>[2x]SETRLSLEDLFRKDFVLHDPEARWINDTDVVYKSENGHVIKLNIETNATTLLLENTTFVTFKASRHSVSPDLKYVLLAYDVKQIFHYSYTASYVIYNIHTREVWELNPPEVEDSVLQYAAWGVQGQQLIYIFENNIYYQPDIKSSSLRLTSSGKEEIIFNGIADWLYEEELLHSHIAHWWSPDGERLAFLMINDSLVPTMVIPRFTGALYPKGKQYPYPKAGQMNPTIKLYVVNLYGPTHTLELMPPDSFKSREYYITMVKWVSNTKTVVRWLNRAQNISILTVCETTTGACSKKYEMTSDTWLSQQNEEPVFSRDGSKFFMTVPVKQGGRGEFHHIAMFLIQSKSEQITVRHLTSGNWEVIKILAYDETTQKIYFLSTESSPRGRQLYSASTEGLLNRQCISCNFMKEQCTYFDASFSPMNQHFLLFCEGPRVPVVSLHSTDNPAKYFILESNSMLKEAILKKKIGKPEIKILHIDDYELPLQLSLPKDFMDRNQYALLLIMDEEPGGQLVTDKFHIDWDSVLIDMDNVIVARFDGRGSGFQGLKILQEIHRRLGSVEVKDQITAVKFLLKLPYIDSKRLSIFGKGYGGYIASMILKSDEKLFKCGSVVAPITDLKLYASAFSERYLGMPSKEESTYQAASVLHNVHGLKEENILIIHGTADTKVHFQHSAELIKHLIKAGVNYTMQVYPDEGHNVSEKSKYHLYSTILKFFSDCLKE

In this paper, we present the crystal structure of human DPP10, a naturally inactive member of the prolyl oligopeptidase family that belongs to the S9B serine protease subfamily. DPP6 and DPP10 are homologous glycosylated, single-pass type II transmembrane proteins that lack the crucial serine residue of the catalytic triad; instead, DPP6 contains an aspartic acid (Asp712) and DPP10 a glycine (Gly651). The Ca2+ binding proteins (KChIPS) and the dipeptidylpeptidase-like proteins (DPPLs) DPP6 (also known as DPPX) and DPP10 (also known as DPPY) associate with the α-subunits of the Kv4 subfamily to form a ternary complex of approximately 750 kDa containing 12 protein molecules (4 copies of each protein per channel). DPP10 and DPP6 both accelerate the activation and inactivation of Kv4.3 channel gating but with distinct biophysical properties.

The extracellular domain (residues 58–796) was expressed as a secreted protein from insect cells, purified and crystallized in space group P212121 with two molecules in the asymmetric unit. The overall structure of DPP10 is very similar to those of DPP6 and DPP4, with Cα-root-mean-square-deviations (r.m.s.d.) of 1.1 Å (for 646 superimposed atoms) and 1.5 Å (for 578 atoms), respectively. Each subunit consists of two domains: an open (no “Velcro” architecture present) β-propeller (residues 82–517, shown in yellow in Fig. 1) consisting of eight blades each built up by four antiparallel β-strands and a classical α/β-hydrolase fold (residues 517–679 and 707–796; shown in red). Additionally, a small-extended arm formed by three helices is inserted between two β-strands of the hydrolase domain (residues 679–707; shown in blue). In our structure, all these asparagine residues with the exception of Asn-90 were found to be glycosylated and well-defined electron densities were observed for the first sugar residues. Similarly to DPP6, DPP10 has three disulfide bonds in the β-propeller (Cys349-Cys356, Cys465-Cys468, Cys475-Cys493) and one in the α/β-hydrolase domain (Cys670-Cys780). DPP10 contains the glutamate residues (Glu-233 and Glu-234), but the serine is replaced by a glycine and the tryptophan residue preceding the serine is replaced by a lysine (changing the sequence to GKGYGG). In DPP10, the entrance is narrowed by the presence of Lys-77, Lys-126 and Glu-763 (channel colored in red). According to a PISA analysis the two DPP10 molecules in the asymmetric unit of the crystal form a symmetric dimer with a total buried surface area of 7300 Å2. The main dimerization interface, which has a two-fold symmetry, between the two chains (1580 Å2 per chain) is formed primarily by residues Pro-262 to Gly-277 and Tyr-282 to Gln-287 of the β-propeller domain, as well as by residues Phe-732 to Ala-745 and Thr-750 to Pro-755 located in the hydrolase domain.>SELDAKLNKLGVDRIAISPYKQWTRGYMEPGNIGNGYVTGLKVDAGVRDKSDNNVLDGIVSYDRAETKNAYIGQINMTTAS[3x];>XFTGVQGRVIGYDILRSPEVDKAKPLFTETQWDGSELPIYDAKPLQDALVEYFGTEQDRRHYPAPGSFIVCANKGVTAERPKNDADMKPGQGYGVWSAIAISFAKDPT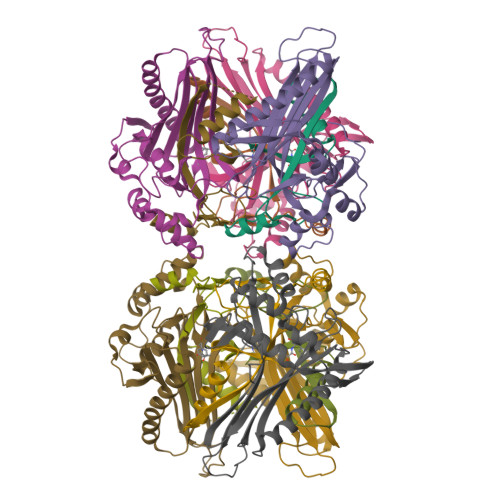KDSSMFVEDAGVWETPNEDELLEYLEGRRKAMAKSIAECGQDAHASFESSWIGFAYTMMEPGQIGNAITVAPYVSLPIDSIPGGSILTPDKDMEIMENLTMPEWLEKMGYKSLSANNALKY[3x]> MGPVTINNFNYNDPIDNNNIIMMEPPFARGTGRYYKAFKITDRIWIIPERYTFGYKPEDFNKSSGIFNRDVCEYYDPDYLNTNDKKNIFLQTMIKLFNRIKSKPLGEKLLEMIINGIPYLGDRRVPLEEFNTNIASVTVNKLISNPGEVERKKGIFANLIIFGPGPVLNENETIDIGIQNHFASREGFGGIMQMKFCPEYVSVFNNVQENKGASIFNRRGYFSDPALILMHQLIYVLHGLYGIKVDDLPIVPNEKKFFMQSTDAIQAEELYTFGGQDPSIITPSTDKSIYDKVLQNFRGIVDRLNKVLVCISDPNININIYKNKFKDKYKFVEDSEGKYSIDVESFDKLYKSLMFGFTETNIAENYKIKTRASYFSDSLPPVKIKNLLDNEIYTIEEGFNISDKDMEKEYRGQNKAINKQAYEEISKEHLAVYKIQMCKSVKAPGICIDVDNEDLFFIADKNSFSDDLSKNERIEYNTQSNYIENDFPINELILDTDLISKIELPSENTESLTDFNVDVPVYEKQPAIKKIFTDENTIFQYLYSQTFPLDIRDISLTSSFDDALLFSNKVYSFFSMDYIKTANKVVEAGLFAGWVKQIVNDFVIEANKSNTMDKIADISLIVPYIGLALNVGNETAKGNFENAFEIAGASILLEFIPELLIPVVGAFLLESYIDNKNKIIKTIDNALTKRNEKWSDMYGLIVAQWLSTVNTQFYTIKEGMYKALNYQAQALEEIIKYRYNIYSEKEKSNINIDFNDINSKLNEGINQAIDNINNFINGCSVSYLMKKMIPLAVEKLLDFDNTLKKNLLNYIDENKLYLIGSAEYEKSKVNKYLKTIMPFDLSIYTNDTILIEMFNKYNSEILNNIILNLRYKDNNLIDLSGYGAKVEVYDGVELNDKNQFKLTSSANSKIRVTQNQNIIFNSVFLDFSVSFWIRIPKYKNDGIQNYIHNEYTIINCMKNNSGWKISIRGNRIIWTLIDINGKTKSVFFEYNIREDISEYINRWFFVTITNNLNNAKIYINGKLESNTDIKDIREVIANGEIIFKLDGDIDRTQFIWMKYFSIFNTELSQSNIEERYKIQSYSEYLKDFWGNPLMYNKEYYMFNAGNKNSYIKLKKDSPVGEILTRSKYNQNSKYINYRDLYIGEKFIIRRKSNSQSINDDIVRKEDYIYLDFFNLNQEWRVYTYKYFKKEEEKLFLAPISDSDEFYNTIQIKEYDEQPTYSCQLLFKKDEESTDEIGLIGIHRFYESGIVFEEYKDYFCISKWYLKEVKRKPYNLKLGCNWQFIPKDEGWTEHHHHHHHHHH;> MNINDNLSINSPVDNKNVVVVRARKTDTVFKAFKVAPNIWVAPERYYGESLSIDEEYKVDGGIYDSNFLSQDSEKDKFLQAIITLLKRINSTNAGEKLLSLISTAIPFPYGYIGGGYYAPNMITFGSAPKSNKKLNSLISSTIPFPYAGYRETNYLSSEDNKSFYASNIVIFGPGANIVENNTVFYKKEDAENGMGTMTEIWFQPFLTYKYDEFYIDPAIELIKCLIKSLYFLYGIKPSDDLVIPYRLRSELENIEYSQLNIVDLLVSGGIDPKFINTDPYWFTDNYFSNAKKVFEDHRNIYETQIEGNNAIGNDIKLRLKQKFRININDIWELNLNYFSKEFSIMMPDRFNNALKHFYRKQYYKIDYPENYSINGFVNGQINVQLSLSDRNQDIINKPEEIINLLNGNNVSLMRSNIYGDGLKSTVDDFYSNYKIPYNRAYEYHFNNSNDSSLDNVNIGVIDNIPEIIDVNPYKENCDKFSPVQKITSTREINTNIPWPINYLQAQNTNNEKFSLSSDFVEVVSSKDKSLVYSFLSNVMFYLDSIKDNSPIDTDKKYYLWLREIFRNYSFDITATQEINTDCGINKVVTWFGKALNILNTSDSFVEEFQNLGPISLINKKENLSMPIIEIYGIPNDMLGLPLNDLNEKLFNIYLKNILYFKKVYFNFLDQWWTEYYSQYFDLICMAKQSILAQEKLIKQIIQNKLQDLFKADISMDKLNLMNLATEKTFIDLSNESQIAINNINDFLNKSAICVFDTNIYPKFISFMEQCINSVNSNVTAFIQKCTNITEDEKLQLIKLNTFMNIDFEFFDIQSIKDLITSETDLIKEEKESDYNLFLFTLQEDNNKVIEDISGKNTLVKYSDSISLVYGVNGDALYLKEPDESVSFSNKAFENGLTNSFSICFWLRNLGEDIITSKLIENKADNCGWEIYFENNGLVFSIVDCNGNEENIYLSDVISKNWYYISISIDRLRNQLLIFINDKLIANQSIEQILNIYSSNTISLVNENNPIYIEGLSILNRSITSEEVVNNYFSYLNNSYIRDISGERLEYNKTYE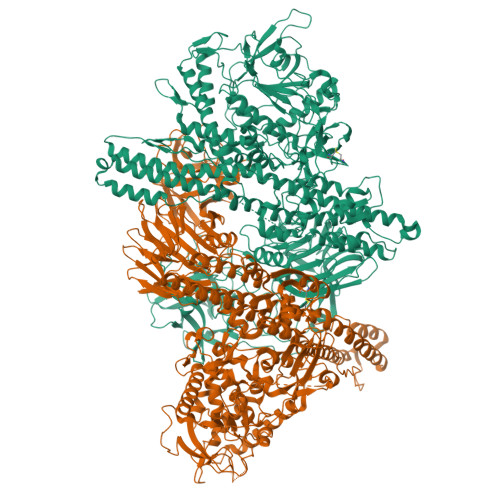LYNYVFPENSLYEVTENNNIYLSIKDTNNLNIQGAKFKLINIDANKQYVQKWDEGVVCLLGDEEKYVDISSENNRIQLVNSKDTAKRIIFNNDIFMPNCLTFAYNNKYLSLSLRDRNYNWMICNNNDNIPKAAHLWALKGI>MEVVSLPRLGEPAPAFEAQTTFGPVKFPDDFKGQWVVLFSHPADFTPVCTTEFVAFAKNYEEFKKRNVQLIGLSVDSNFSHIAWVMNIKEKFGIEIPFPIIADHNMEVAKKYGMIHPAQSTTFTVRALFVIDDKGILRAMIYYPLTTGRNIREVIRLVDALQTADREGVATPADWVPEPQTWEFTEENTKVIVPPPTTYEDAVKRLQEGYECADWYICKKKVA[5x];>MEVVSLPRLGEPAPAFEAQTTFGPVKFPDDFKGQWVVLFSHPADFTPVCTTEFVAFAKNYEEFKKRNVQLIGLSVDSNFSHI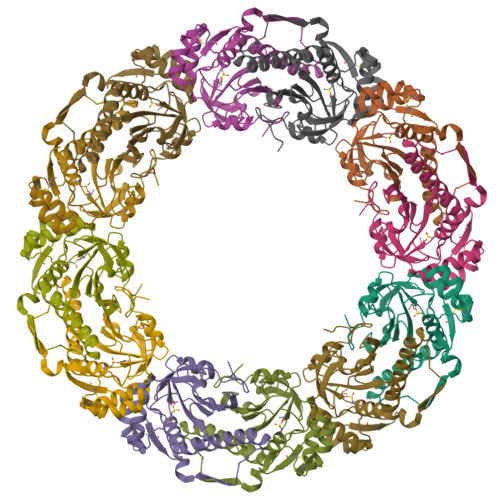AWVMNIKEKFGIEIPFPIIADHNMEVAKKYGMIHPAQSTTFTVRALFVIDDKGILRAMIYYPLTTGRNIREVIRLVDALQTADREGVATPADWVPEPQTWEFTEENTKVIVPPPTTYEDAVKRLQEGYECADWYICKKKV[7x]> SNAAMSQKHLQINQTFEELRLVTQDTENELKKLQQTQEYFIIQYQESLRIQAQFAQLAQLSPQERLSRETALQQKQVSLEAWLQREAQTLQQYRVELAEKHQKTLQLLRKQQTIILDDELIQWKRRQQLAGNGGPPEGSLDVLQSWCEKLAEIIWQNRQQIRRAEHLCQQLPIPGPVEEMLAEVNATITDIISALVTSTFIIEKQPPQVLKTQTKFAATVRLLVGGKLNVHMNPPQVKATIISEQQAKSLLKNENTRNECSGEILNNCCVMEYHQATGTLSAHFRNMSLKRIKRADRRGAESVTEEKFTVLFESQFSVGSNELVFQVKTLSLPVVVI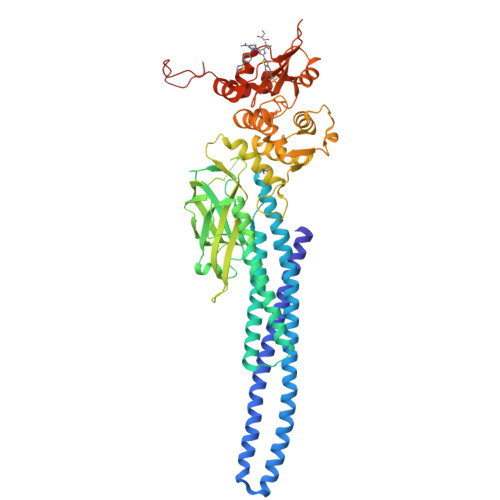VHGSQDHNATATVLWDNAFAEPGRVPFAVPDKVLWPQLCEALNMKFKAEVQSNRGLTKENLVFLAQKLFNNSSSHLEDYSGLSVSWSQFNRENLPGWNYTFWQWFDGVMEVLKKHHKPHWNDGAILGFVNKQQAHDLLINKPDGTFLLRFSDSEIGGITIAWKFDSPERNLWNLKPFTTRDFSIRSLADRLGDLSYLIYVFPDRPKDEVFSKYYTPVLAKAVDGYVKPQIKQVVPE> MRGSHHHHHHGSSYQIAVLAGDGIGPEVMAEARKVLKAVEAR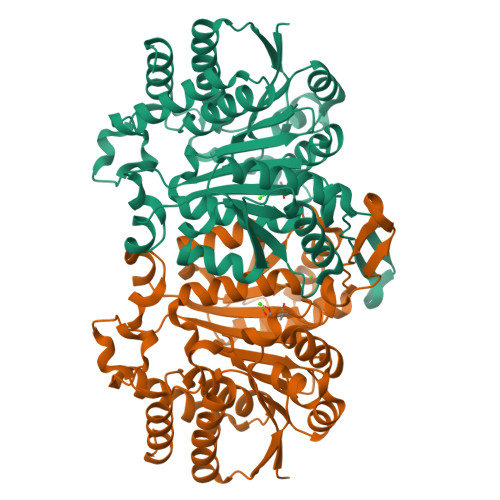FGLNIEYTEYDVGGIAIDNHGCPLPEATLKGCEAADAILFGSVGGPKWEKLPPNEQPERGALLPLRGHFELFCNLRPAKLHDGLEHMSPLRSDISARGFDVLCVRELTGGIYFGKPKGRQGEGESEEAFDTMRYSRREISRIARIAFEAARGRRKKVTSVDKANVLACSVLWRQVVEEVAVDFPDVELEHIYIDNATMQLLRRPDEFDVMLCSNLFGDILSDEIAMLTGSMGLLSSASMNSTGFGLFEPAGGSAPDIAGKGIANPIAQILSAALMLRHSLKQEEAASAIERAVTKALNSGYLTGELLSSDQRHKAKTTVQMGDFIADAVKAGV>MKINDDIKELILEYMSRYFKFENDFYKLPGIKFTDANWQKFKNGGTDIEKMGAARVNAMLDCLFDDFELAMIGKAQTNYYNDNSLKMNMPFYTYYDMFKKQQLLKWLKNNRDDVIGGTGRMYTASGNYIANAYLEVALESSSLGSGSYMLQMRFKDYSKGQEPIPSGRQNRLEWIENNLENIR[2x];> MSDLVLGLDIGIGSVGVGILNKVTGEIIHKNSRIFPAAQAENNLVRRTNRQGRRLTRRKKHRRVRLNRLFEESGLITDFTKISINLNPYQLRVKGLTDELSNEELFIALKNMVKHRGISYLDDASDDGNSSIGDYAQIVKENSKQLETKTPGQIQLERYQTYGQLRGDFTVEKDGKKHRLINVFPTSAYRSEALRILQTQQEFNPQITDEFINRYLEILTGKRKYYHGPGNEKSRTDYGRYRTSGETLDNIFGILIGKCTFYPDEFRAAKASYTAQEFNLLNDLNNLTVPTETKKLSKEQKNQIINYVKNEKAMGPAKLFKYIAKLLSCDVADIKGYRIDKSGKAEIHTFEAYRKMKTLETLDIEQMDRETLDKLAYVLTLNTEREGIQEALEHEFADGSFSQKQVDELVQFRKANSSIFGKGWHNFSVKLMMELIPELYETSEEQMTILTRLGKQKTTSSSNKTKYIDEKLLTEEIYNPVVAKSVRQAIKIVNAAIKEYGDFDNIVIEMARETNEDDEKKAIQKIQKANKDEKDAAMLKAANQYNGKAELPHSVFHGHKQLATKIRLWHQQGERCLYTGKTISIHDLINNSNQFEVDHILPLSITFDDSLANKVLVYATANQEKGQRTPYQALDSMDDAWSFRELKAFVRESKTLSNKKKEYLLTEEDISKFDVRKKFIERNLVDTRYASRVVLNALQEHFRAHKIDTKVSVVRGQFTSQLRRHWGIEKTRDTYHHHAVDALIIAASSQLNLWKKQKNTLVSYSEDQLLDIETGELISDDEYKESVFKAPYQHFVDTLKSKEFEDSILFSYQVDSKFNRKISDATIYATRQAKVGKDKADETYVLGKIKDIYTQDGYDAFMKIYKKDKSKFLMYRHDPQTFEKVIEPILENYPNKQINEKGKEVPCNPFLKYKEEHGYIRKYSKKGNGPEIKSLKYYDSKLGNHIDITPKDSNNKVVLQSVSPWRADVYFNKTTGKYEILGLKYADLQFEKGTGTYKISQEKYNDIKKKEGVDSDSEFKFTLYKNDLLLVKDTETKEQQLFRFLSRTMPKQKHYVELKPYDKQKFEGGEALIKVLGNVANSGQCKKGLGKSNISIYKVRTDVLGNQHIIKNEGDKPKL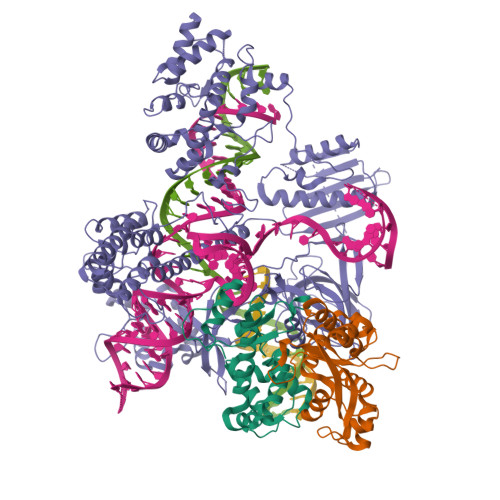DF>GKKQKTRTVFSSTQLCVLNDRFQRQKYLSLQQMQELSNILNLSY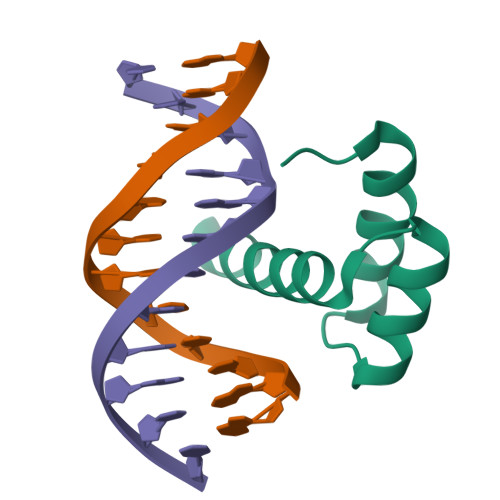KQVKTWFQNQRMKSKRWQKNNWPKNS[2x]> MENTENSVDSKSIKNLEPKIIHGSESMDSGIS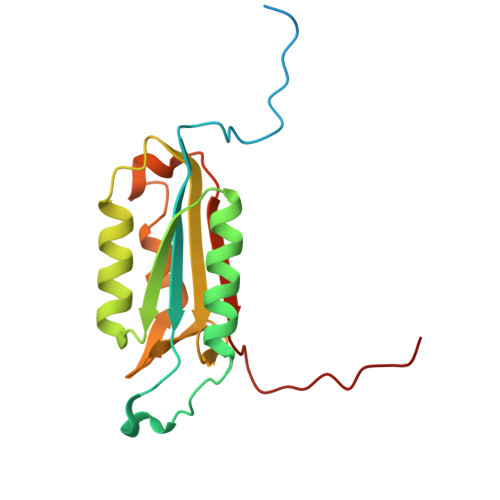LDNSYKMDYPEMGLCIIINNKNFHKSTGMTSRSGTDVDAANLRETFRNLKYEVRNKNDLTREEIVELMRDVSKEDHSKRSSFVCVLLSHGEEGIIFGTNGPVDLKKITNFFRGDRCRSLVGKPKLFIIQACRGTELDCGIETD>MSYQSTIVPVELHSFEDAQVIGGAFRDGDAVVFDMSLLSREEARRIVDFAAGL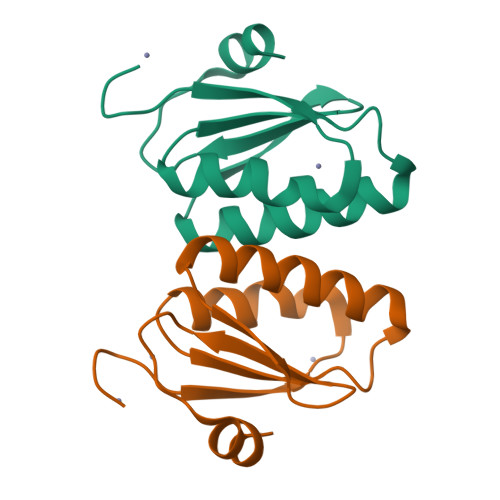CFALRGKMQKIDSVTFAVVPELSNISTSELERAARIR[2x]>[4x]MDRMKIE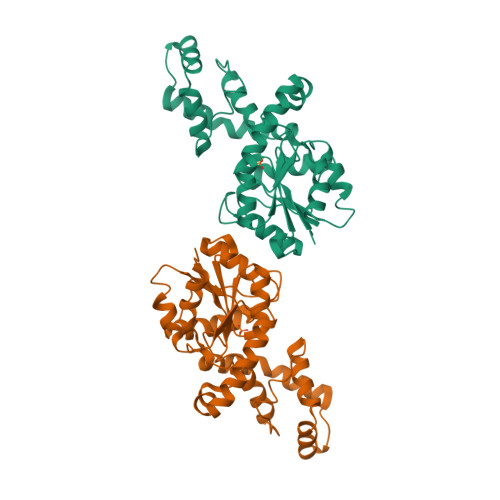AVIFDWAGTTVDYGCFAPLEVFMEIFHKRGVAITAEEARKPMGLLRIDHVRALTEMPRIASEWNRVFRQLPTEADIQEMYEEFEEILFAILPRYASPINGVKEVIASLRERGIKIGSTTGYTREMMDIVAKEAALQGYKPDFLVTPDDVPAGRPYPWMCYKNAMELGVYPMNHMIKVGDTVSDMKEGRNAGMWTVGVILGSSELGLTEEEVENMDSVELREKIEVVRNRFVENGAHFTIETMQELESVMEHIEKQELIIS>[3x]MASWSHPQFEKGAETAVPNSSSVPGDPSSMGRQSNVLFIIIDQLRADCLWGALADHVELPHLRALAQDAVSFRRHYSVTNPCGPSRASILTGQYAMNHRSVRNGTPLRHDTPNIATEMRKAGYLPLLFGYTDTSQDPRAYDANDPALKTYEFPMRGFHEVTEMRLEMSYPWQSHLKNRGYAFDDYAQVYVPRPDADGTPRLNGPAMYRAEDSDTAFLTDQFLANMPAWAGQNWFAHLTYIRPHPPLVA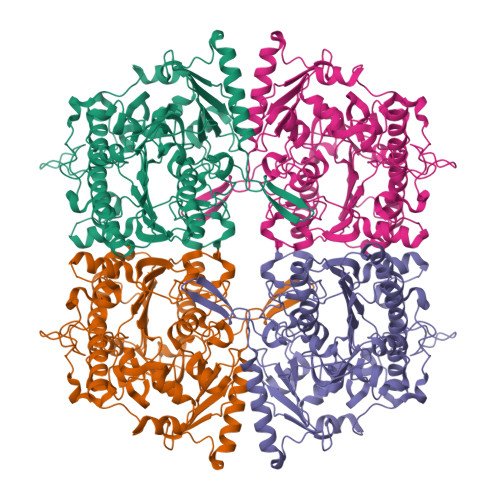PAPYNTMYDPAKLPLPARLPGRDDETAEHPFFGPATRYSSPASFVLGFPDLEPTDETIQTLRAVYLGLATEVDTHIGRVIAHLKETGQYDDTLIVVTADHGEMLGDRHSWGKMTVYDAAYHTPLIIRAPGCKPGHVVEAPTESIDLMPTILDWVGQEIPNAVDGRSLRPFLTGEAPSDWRQYSFSELDISEPLDPTLWQQEFGFGPSAGAVAILRDARFTLVEFAADLPPMLFDHQGEGEFRNVAGDPAHAADLARLSRQMLRHRMRNMDHTLSLCSITHEGARTQRRYD>HHHHHHMEPACKYDFATSVLFTEAELHTRMRGVAQRIADDYSNCNLKPLENPLVIVSVLKGSFVFTADMVRILGDFGVPTRVEFLRASSYGHDTKSCGRVDVKADGLCDIRGKHVLVLEDILDTALTLREVVDSLKKSEPASIKTLVAIDKPGGRKIPFT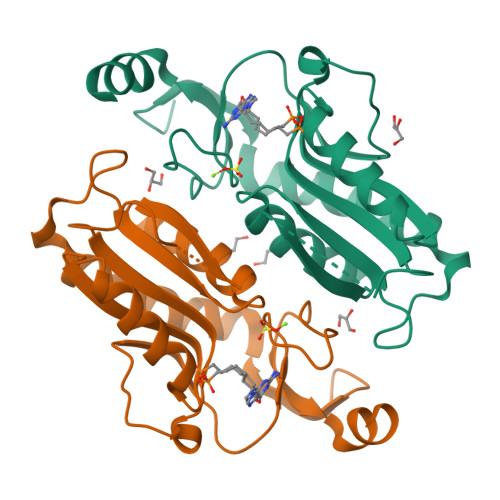AEYVVADVPNVFVVGYGLDYDQSYREVRDVVILKPSVYETWGKELERRKAAGEAKR[2x]> SNAMQQTKTLIVALATMLAGVTAAQAEIKIGITMSASGPGAALGQPQSKTVAALPKEIGGEKVTYFALDDESDPTKAAQNARKLLSEEKVDVLIGSSLTPVSLPLIDIAAEAKTPLMTMAAAAILVAPMDERRKWVYKVVPNDDIMAEAIGKYIAKTGAKKVGYIGFSDAYGEGYYKVLAAAAPKLGFELTTHEVYARSDASVTGQVLKIIATKP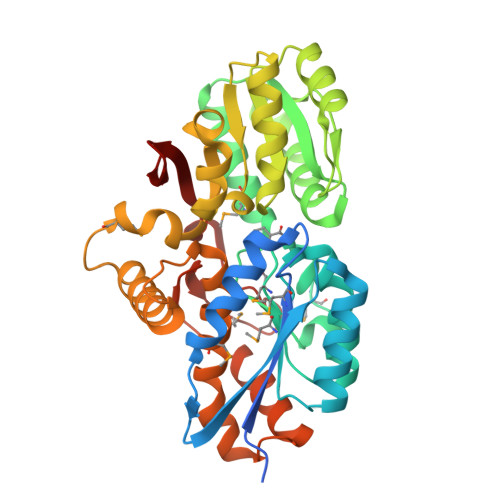DAVFIASAGTPAVLPQKALRERGFKGAIYQTHGVATEEFIKLGGKDVEGAIFAGEAFSGAEDMPADSPFRKVKARFVDAYKAANGGAAPTIFGVHLWDSMTLVENAIPAALKAAKPGTPEFRAAIRDQIEKSKDLALNNGLSNMTPDNHNGYDERSAFLIEIRDGAFRLKQ> GPHMVKHPLNTAWTLWYTKPAVDKSESWSDLLRPVTSFQTVEEFWAII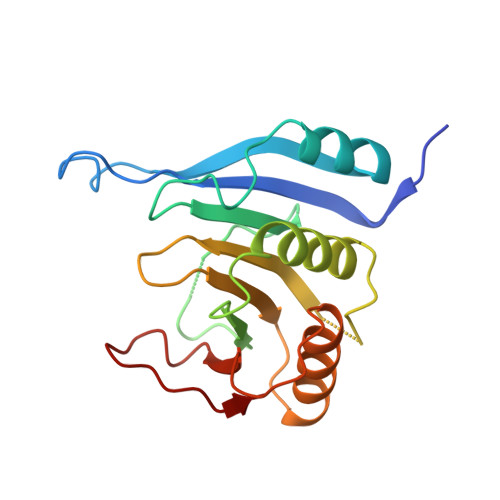QNIPEPHELPLKSDYHVFRNDVRPEWEDEANAKGGKWSFQLRGKGADIDELWLRTLLAVIGETIDEDDSQINGVVLSIRKGGNKFALWTASEDKEPLLRIGGKFKQVLALTDDGHLEFFPHSSANGRHPQPSITL>TKSFTLPILTISEMTNSRFPIPIEQLYTAPNETNVVQCQNGRCTLDGELQGTTQLLSSAICSYRGRTLANNDSWDQNLLQLSYPNGASYDPTDEVPAPLGTQDFSGILYGVLTQDNVTEGTGEAKNAKGIYISTTSGKFTPKIGSIGLHSITGDVHHNQQSRFTPVGIAVNENTPFKQWVLPHYSGSLALNTNLAPAVAPTFPGEQLLFFRSRVPCVQGLHGQDAFIDCLLPQEWVNHFYQEAAPSQTDVALIRFVNP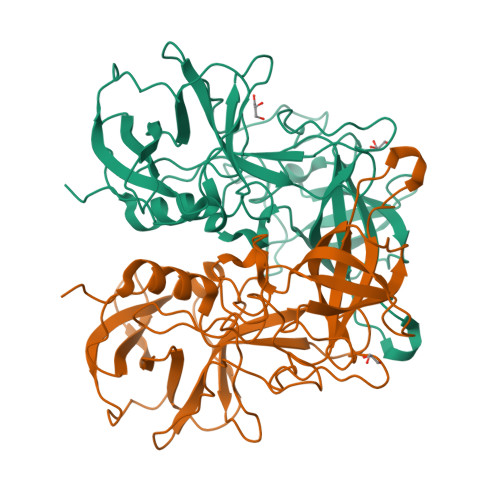DTGRTLFEAKLHRSGFITVSHTGNYPLVIPPNGHFRFDSWVNQFYSLAPM[4x]N-(2-amino-1H-benzimidazol-5-yl)-2-[3-[(2-amino-2-oxoethyl)-methylsulfonylamino]phenyl]acetamide 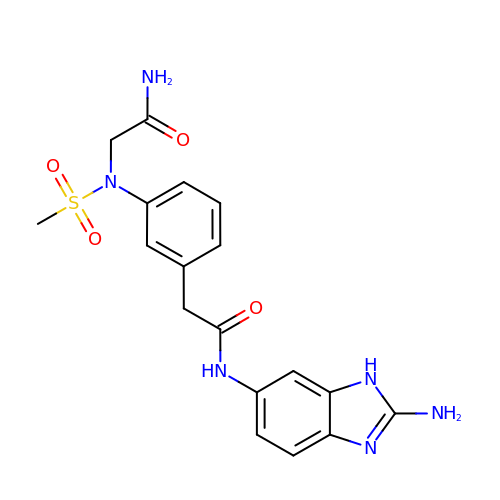| C18 H20 N6 O4 S | HJSXBGSJJLBQNX-UHFFFAOYSA-N1-benzyl-1H-imidazo[4,5-b]pyridine | C13 H11 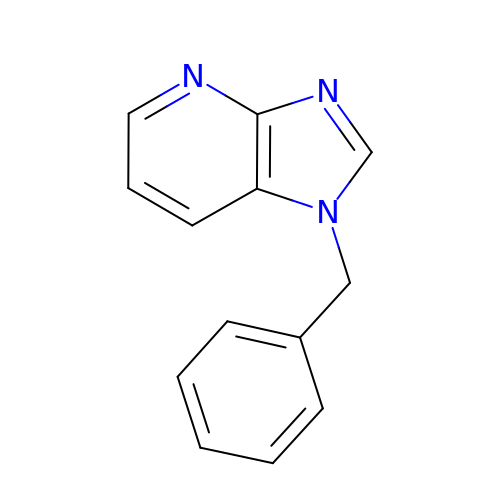N3 | AHFFRONGQSRICB-UHFFFAOYSA-N>[2x]SNAMKTLEKVNYKGFIWPLAVGIVLWLITPWRPGGLSVQAWEMFAIFVATIVGCITKPLPIGGTTLLGMVVTVLVGLAPVKDVVNSKGVVIQTGILSSFGNSAAWLIAMAFIMAHGISKTGLGNRVAYVMIEKFGKRSIGIGYAITGLELMMGALIPSNSARTGGVTWPVVESISKSYDSKPNDPSRKKIGAYLDFMAFHANILSTALFITGAAPNLVAQQMAAQKGYQMSWVSWFWAALVPVLVATVIIPLVIYKMYPPEVKETPNAKNWADDKLKEMGPISKPEKIMATVFCLAILLWVLSGFFKIPQLDSAFVAFLAVTLLLITGVLSMEDALHETGAWNILIWLSILIFMAGKLISYGFIAWFAKFIQSEVHGINWGLVLVVLILLMFYTHYFFASGTAHMTALYLPFLTVATAMGAPLGLSAMLLAFTGVINASTTHYANGPASILATTGYVKQSEWWKMNFILGLIYMVIFGIVGTIWMKIIGIW

The mammalian SLC13 proteins are members of the larger divalent-anion sodium symporter (DASS) family. DASS proteins typically have a molecular weight of 45–65 kDa and form obligate homodimers. Each protomer consists of a scaffold and a transport domain. Structural information, along with cross-linking and computer modeling, indicates that DASS proteins operate in an elevator-type transport mechanism (Reyes et al., 2009; Drew and Boudker, 2016; Garaeva and Slotboom, 2020).

We also solved a 2.85 Å X-ray structure of LaINDY in the presence of both malate and αKG, using the LaINDY-αKG cryo-EM structure as the search model for molecular replacement. The structures of LaINDY determined in malate, αKG and in the malate/αKG mixture are in an outward-facing, substrate-bound (Co-S) state. The architecture of the LaINDY binding site is similar to that of VcINDY. Notably, within the binding site, density corresponding to substrate is seen in the X-ray omit map of LaINDY-malate-αKG, and in the LaINDY-αKG cryo-EM difference map, in a similar mode to substrate binding in VcINDY. All three Co-S structures are not only similar to each other but, importantly, also to the LaINDY Co apo structure, with pairwise r.m.s.d.s of 0.41–0.52 Å, indicating that substrate binding introduces little conformational change. In contrast to the similarity at the substrate binding site, major differences between LaINDY and VcINDY are seen at the cation binding sites. At the Na1 site of VcINDY, an arginine (Arg159) is found in LaINDY, stabilized by a salt bridge with Glu146. Similarly, a histidine (His392) in LaINDY is located at the equivalent of the VcINDY Na2 site, with another histidine (His401) located 4 Å on its extracellular side. Based on these well enclosed and sterically occupied cation binding sites, it is unlikely that sodium ions bind to LaINDY as Na1 and Na2 do in VcINDY. Rather, we hypothesize these two positively-charged residues in exchangers act as permanent surrogates of the Na+ ions in cotransporters.>[4x]MPKRTDIKSILILGAGPIVIGQACEFDYSGAQACKALREEGYRVILVNSNPATIMTDPEMADATYIEPIHWEVVRKIIEKERPDAVLPTMGGQTALNCALELERQGVLEEFGVTMIGATADAIDKAEDRRRFDVAMKKIGLETARSGIAHTMEEALAVAADVGFPCIIRPSFTMGGSGGGIAYNREEFEEICARGLDLSPTKELLIDESLIG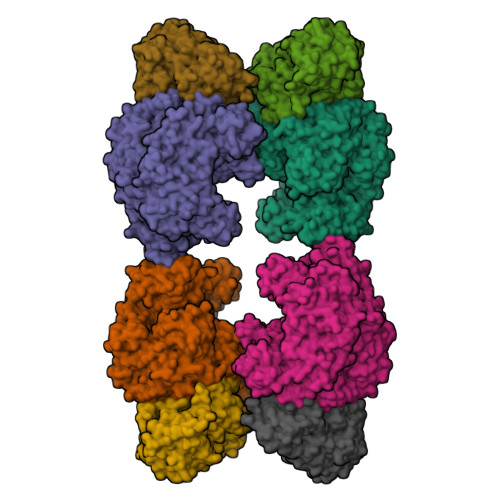WKEYEMEVVRDKNDNCIIVCSIENFDAMGIHTGDSITVAPAQTLTDKEYQIMRNASMAVLREIGVETGGSNVQFAVNPKNGRLIVIEMNPRVSRSSALASKATGFPIAKVAAKLAVGYTLDELMNDITGGRTPASFEPSIDYVVTKIPRFNFEKFAGANDRLTTQMKSVGEVMAIGRTQQESLQKALRGLEVGATGFDPKVSLDDPEALTKIRRELKDAGADRIWYIADAFRAGLSVDGVFNLTNIDRWFLVQIEELVRLEEKVAEVGITGLNADFLRQLKRKGFADARLAKLAGVREAEIRKLRDQYDLHPVYKRVDTCAAEFATDTAYMYSTYEEECEANPSTDREKIMVLGGGPNRIGQGIEFDYCCVHASLALREDGYETIMVNCNPETVSTDYDTSDRLYFEPVTLEDVLEIVRIEKPKGVIVQYGGQTPLKLARALEAAGVPVIGTSPDAIDRAEDRERFQHAVERLKLKQPANATVTAIEMAVEKAKEIGYPLVVRPSYVLGGRAMEIVYDEADLRRYFQTAVSVSNDAPVLLDHFLDDAVEVDVDAICDGEMVLIGGIMEHIEQAGVHSGDSACSLPAYTLSQEIQDVMRQQVQKLAFELQVRGLMNVQFAVKNNEVYLIEVNPRAARTVPFVSKATGVPLAKVAARVMAGKSLAEQGVTKEVIPPYYSVKEVVLPFNKFPGVDPLLGPEMRSTGEVMGVGRTFAEAFAKAQLGSNSTMKKHGRALLSVREGDKERVVDLAAKLLKQGFELDATHGTAIVLGEAGINPRLVNKVHEGRPHIQDRIKNGEYTYIINTTSGRRAIEDSRVIRRSALQYKVHYDTTLNGGFATAMALNADATEKVISVQEMHAQIK;>MIKSALLVLEDGTQFHGRAIGATGSAVGEVVFNTSMTGYQEILTDPSYSRQIVTLTYPHIGNVGTNDADEESSQVHAQGLVIRDLPLIASNFRNTEDLSSYLKRHNIVAIADIDTRKLTRLLREKGAQNGCIIAGDNPDAALALEKARAFPGLNGMDLAKEVTTAEAYSWTQGSWTLTGGLPEAKKEDELPFHVVAYDFGAKRNILRMLVDRGCRLTIVPAQTSAEDVLKMNPDGIFLSNGPGDPAPCDYAITAIQKFLETDIPVFGICLGHQLLALASGAKTVKMKFGHHGGNHPVKDVEKNVVMITAQNHGFAVDEATLPANLRVTHKSLFDGTLQGIHRTDKPAFSFQGHPEASPGPHDAAPLFDHFIELIEQYRKTAK[4x]> L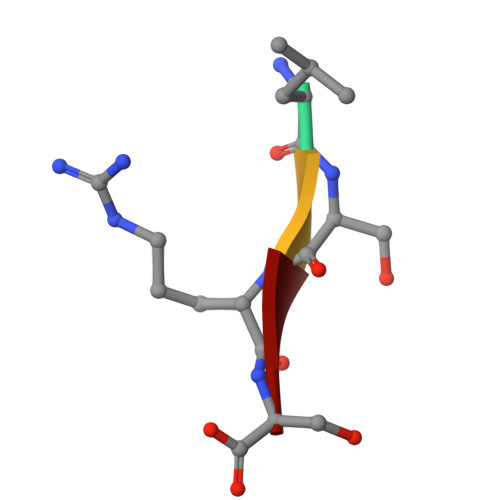SRS> HMIKLSNITKVFHQGTRTIQALNNVSLHVPAGQIYGVIGASGAGKSTLIRCVNLLERPTEGSVLVDGQELTTLSESELTKARRQIGMIFQHFNLLSSRTV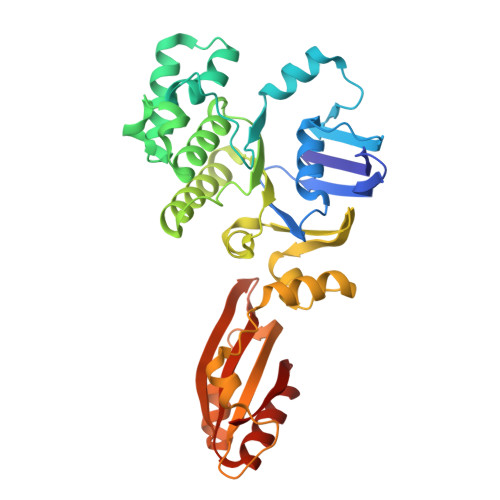FGNVALPLELDNTPKDEVKRRVTELLSLVGLGDKHDSYPSNLSGGQKQRVAIARALASNPKVLLCDQATSALDPATTRSILELLKDINRRLGLTILLITHEMDVVKRICDCVAVISNGELIEQDTVSEVFSHPKTPLAQKFIQSTLHLDIPEDYQERLQAEPFTDCVPMLRLEFTGQSVDAPLLSETARRFNVNNAIISAQMDYAGGVKFGIMLTEMHGTQQDTQAAIAWLQEHHVKVEVLGYV>GQDKPIRTEESLEGTVIYKKTTTFEVDGYTYQCDVDDGSQFVTLYNKENKLTYEKIVYKDTGKTYIGSWSSNVIEYDRFMSQQADFIVDQAFTKAMADEIGKTELMITMLLSPNTGEVMEVNFNFFTFEPYAKVPLHVYREIEVKLKEQIHFKPIEEGKQLNY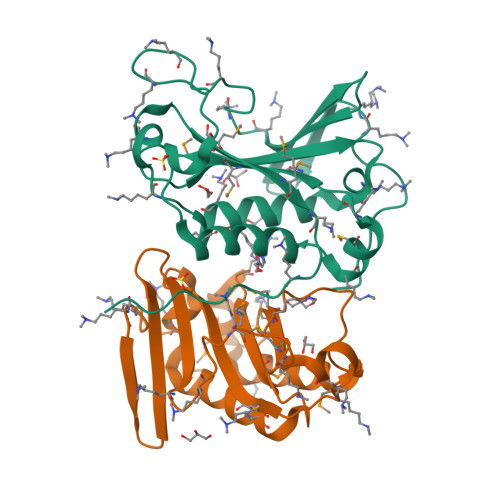IMLAWMQKPQGKLPPLPPPGSLM[2x]2-carbazol-9-yl-N-(2-chloranyl-6-cyano-phenyl)ethanamide | C21 H14 Cl N3 O | 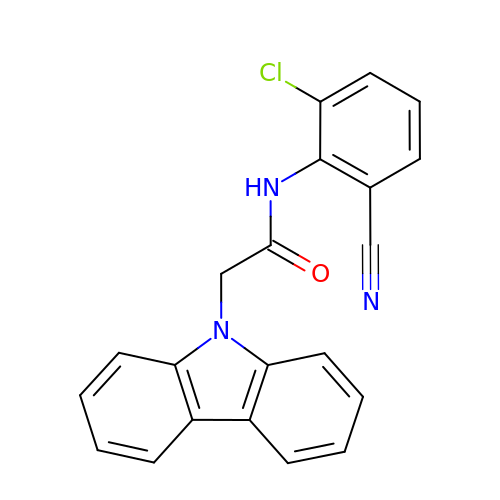ZDAKKNHUWVTCRS-UHFFFAOYSA-N> QEHEPIGAQDERLSTLIHQRM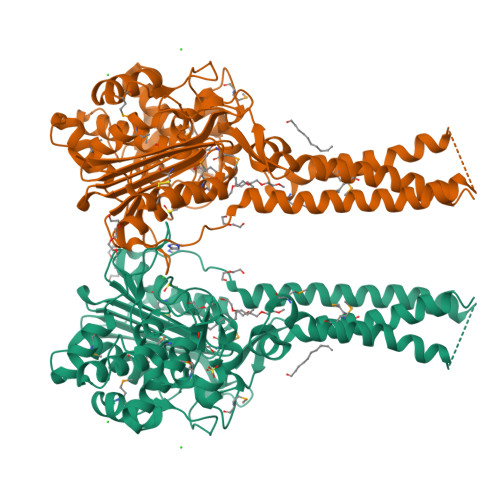QEAKVPALSVSVTIKGVRQRFVYGVADVASQKANTLDTVYELGAMSKAFTGLVVQILIQEGRLRQGDDIITYLPEMRLNYQGKPASLTVADFLYHTSGLPFSTLARLENPMPGSAVAQQLRNENLLFAPGAKFSYASANYDVLGAVIENVTGKTFTEVIAERLTQPLGMSATVAVKGDEIIVNKASGYKLGFGKPVLFHAPLARNHVPAAYIHSTLPDMEIWIDAWLHRKALPATLREAMSNSWRGNSDVPLAADNRILYASGWFIDQNQGPYISHGGQNPNFSSCIALRPDQQIGIVALANMNSNLILQLCADIDNYLRIGKYADGAGDAITATDTLFVYLTLLLCFWGAVVVVRGAFRVYRATAHGPGKQQRLRLRVRDYIIALAVPGLVAAMLYVAPGIMSPGLDWRFILVWGPSSVLAIPFGMILLAFVLTLNHQIKRILLHNKEWDDEHHHHHH> HGYVQNIVIDGESYSGYIVTQFPYESNPPAVIGWATTATDLGYVDPTEYTNADIICHKNATPGALSAPVAAGGTVELQWTTWPDSHHGPVISYLANCNGNCSTVDKTKLDFVKIDASGLIDDTTVPGTWASDQLIAANNSWTVTIPETIAPGNYVLRHEIIALHSAENTDGAQNYPQCINLEITGSGTASPTGTPGEELY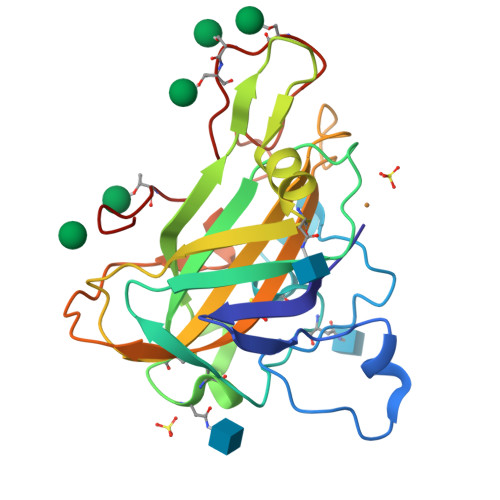TPTDPGILVNIYQSLSTYVIPGPTLWSGAA> SNRFYLLTLTSNQDESITLAIDVEDMVAVAYQPAGSHESYFFLNAPQIAFHTLFTDTHQNVLNFDNTFKSLENAAGTTRQTIVLGVDPLDFAISNLFNADPKLLPLSFLVIIQMVLEASKFRFIEQSVAYSF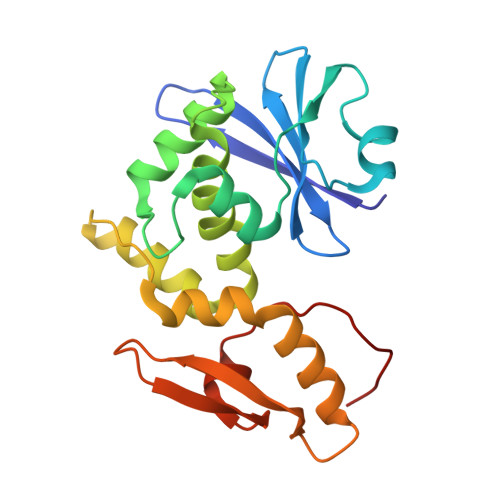KNEKTFLPDLAIVSLEDNWSEISLQIQASTSLQGLFGSVVELYNSNNELIEVDSIYYPIILANVALQLYHCQVSTGD>GAASMSDDLVKILVLGPSKSGKSTVTNFLAGTRDTPTKEYHETNPLRVLEVEIALDDTRRSGRQAAGLKKAVVQLWDVGGSSKHQAGWPAIASNADGIIYVFNPEVKGSEKELLLWYKNFALNQDELDDDNNFKMRVTDGHSLIFSHHSSLPEFAVGDNAIPPMPKQLQGIR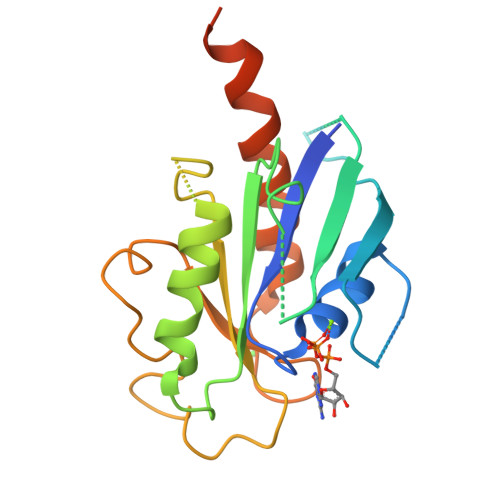ALETSLDYQSDNFKEAFDALVEQIIASRLAAEENDLLQKEREAKDYPRLKR[2x]N-(3-carboxypropanoyl)-L-valyl-N-[(1S)-2-phenyl-1-phosphonoethyl]-L-prolinamide 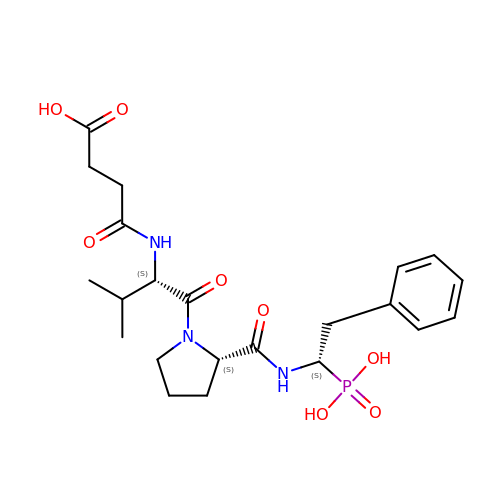| C22 H32 N3 O8 P | KPGFVOVOBVGIMY-QRFRQXIXSA-N> ALGLLAPLRETKSTNPASRVME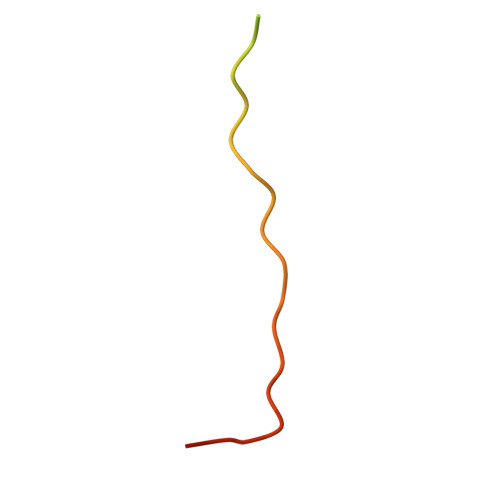MEPETMETKSVIDSRV>[3x]QVYPIGTEK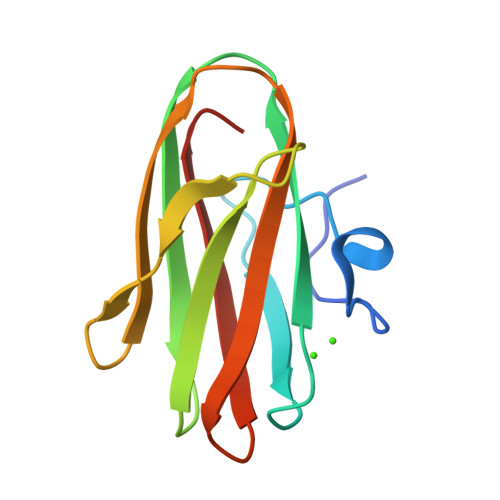EPNNSKETASGPIVPGIPVSGTIENTSDQDYFYFDVITPGEVKIDINKLGYGGATWVVYDENNNAVSYATDDGQNLSGKFKADKPGRYYIHLYMFNGSYMPYRINIEGSVGR> DDSQIKKADATSVAVDASISAFPKKMGPPQWPFSTQYELIGKGVRCVSSI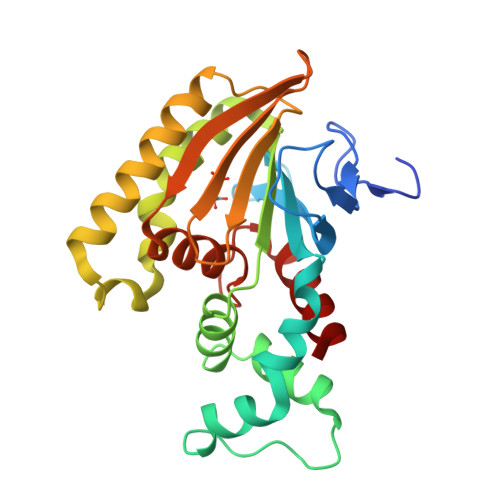TFKAYGLGIYVAAEDKHLVSEVLDSKFLSQAFIDTAAPPSPENSHQDNLRAALNDPAKAPILINNLLDSGIRLMSKNTPIKAGSFKLLMDGTKKSVLKNPDSQSQDKDRLEAGFQELHDCFRSVKGLVARDDDFFIELNKDCSMNLSYYARKKDEFVILGTVKEPLIGKLLFAHYLAAVDPPSPEARKEVIDALVSLS>[2x]MADKLFINALKKKFEESPEEKKTTFYTLGGWKQSERKTEFVNAGKEVAEKRGIPQYNPDIGTPLGQRVLMPYQVSTTDTYVEGDDLHFVNNAAMQQLWDDIRRTVIVGLNHAHAVIEKRLGKEVTPETITHYLETVNHAMPGAAVVQEHMVETHPALVADSYVKVFTGNDEIADEIDPAFVIDINKQFPEDQAETLKAEVGDGIWQVVRIPTIVSRTCDGATTSRWSAMQIGMSMISAYKQAAGEAATGDFAYAAKHAEVIHMGTYLPVRRARGENEPGGVPFGYLADICQSSRVNYDDPVRVSLDVVATGAMLYDQIWLGSYMSGGVGFTQYATAAYTDNILDDFTYFGKEYVEDKYGLCEAPNTMDTVLDIATEVTFYGLEQYEEYPALLEDQFGGSQRAAVVAAAAGCSTAFATGNAQTGLS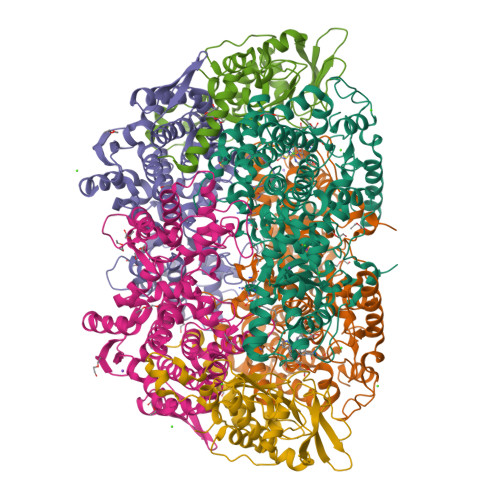GWYLSMYLHKEQHSRLGFYGYDLQDQCGASNVFSIRGDEGLPLELRGPNYPNYAMNVGHQGEYAGISQAPHAARGDAFVFNPLVKIAFADDNLVFDFTNVRGEFAKGALREFEPAGERALITPAK;>[2x]MAKFEDKVDLYDDRGNLVEEQVPLEALSPLRNPAIKSIVQGIKRTVAVNLEGIENALKTAKVGGPACKIMGRELDLDIVGNAESIAAAAKEMIQVTEDDDTKVELLGGGKRALVQVPSARFDVAAEYSAAPLVTATAFVQAIINEFDVSMYDANMVKAAVLGRYPQSVEYMGANIATMLDIPQKLEGPGYALRNIMVNHVVATTLKNTLQAAALSTILEQTAMFEMGDAVGAFERMHLLGLAYQGMNADNLVFDLVKANGKEGTVGSVIADLVERALEDGVIKVEKELTDYKVYGTDDLAMWNAYAAAGLMAATMVNQGAARAAQGVSSTLLYYNDLIEFETGLPSVDFGKVEGTAVGFSFFSHSIYGGGGPGIFNGNHIVTRHSKGFAIPCVAAAMALDAGTQMFSPEATSGLIKEVFSQVDEFREPLKYVVEAAAEIKNEI;>[2x]MAQYYPGTSKVAQNRRNFCNPEYELEKLREISDEDVVKILGHRAPGEEYPSVHPPLEEMDEPEDAIREMVEPIDGAKAGDRVRYIQFTDSMYFAPAQPYVRSRAYLCRYRGADAGTLSGRQIIETRERDLEKVSKELLETEFFDPARSGVRGKSVHGHSLRLDEDGMMFDMLRRQIYNKDTGKVEMVKNQIGDELDEPVDLGEPLDEETLMDKTTIYRVDGEAYRDDVEAVEIMQRIHVLRSQGGYNPE> GSHMASMKKKGSVVIVGRINLSGDTAYAQQTRGEEGCQETSQTGRDKNQVEGEVQIVSTATQTFLATSINGVLWTVYHGAGTRTIASPKGPVTQMYTNVDKDLVGWQAPQGSRSLTPCTCGSSDLYLVTRHADVIPVRRRGDSRGSLLSPRPISYLKGSSGGPLLCPA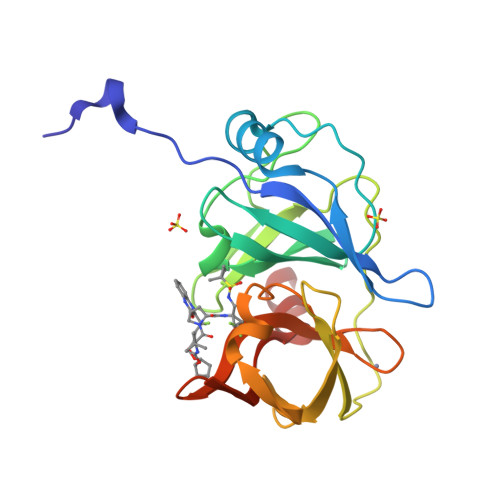GHAVGIFRAAVCTRGVAKAVDFIPVESLETTMRSP~{N}-[4-bromanyl-3-[(3~{S})-3-methylpyrrolidin-1-yl]sulfonyl-phenyl]-2-[(4~{R})-4-cyclopropyl-4-methyl-2,5-bis(oxidanylidene)imidazolidin-1-yl]ethanamide 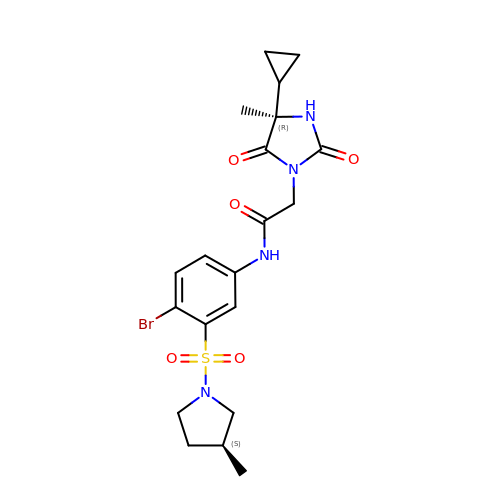| C20 H25 Br N4 O5 S | XHAYAQCABOVSNX-FKIZINRSSA-N>GSFTMDHYLDIRLRPDPEFPPAQLMCVLFGKLHQALVAQGGDRIGVSFPDLDESRSRLGERLRIHASADDLRALLARPWLEGLRDHLQFGEPAVVPHPTPYRQVSRVQAKSNPERLRRRLMRRHDLSEEEARKRIPDTVARTLDL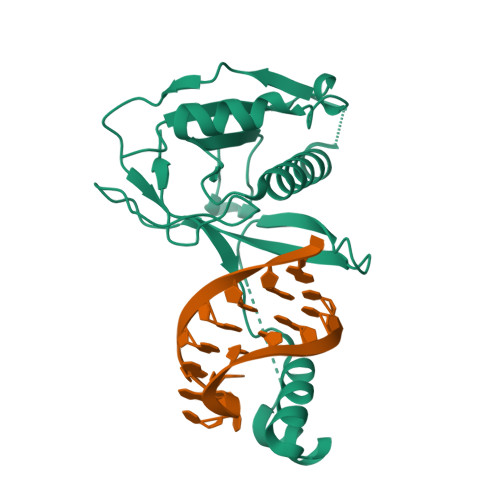PFVTLRSQSTGQHFRLFIRHGPLQVTAEEGGFTCYGLSKGGFVPWF[2x]> TVGAVALDLDGNLAAATSTGGMTN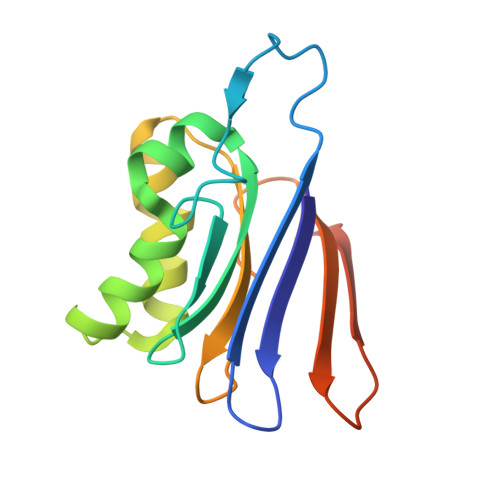KLPGVVGPWPLVGAGCYANNASVAVSCTGTGEVFIRALAAYDIAALMDYGGLSLAEACERVVMEKLPALGGSGGLIAIDHEGNVALPFNTEGMYRAWGYAGDTPTTGIYREKGDTVATQ>[2x]HHHHHHMASSAQDGNNPLFSPYKMGKFNLSHRVVLAPMTRCRALNNIPQAALGEYYEQRATAGGFLITEGTMISPTSAGFPHVPGI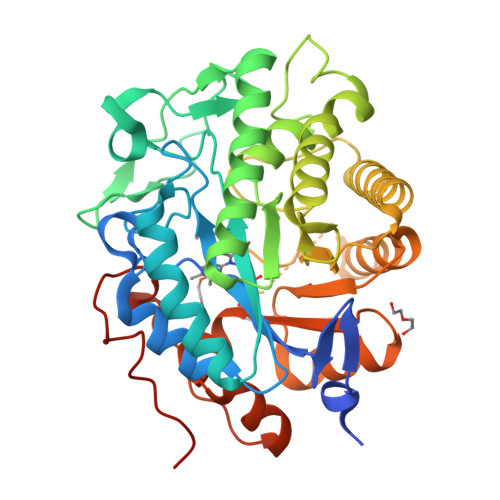FTKEQVREWKKIVDVVHAKGAVIFCQLWHVGRASHEVYQPAGAAPISSTEKPISNRWRILMPDGTHGIYPKPRAIGTYEISQVVEDYRRSALNAIEAGFDGIEIHGAHGYLIDQFLKDGINDRTDEYGGSLANRCKFITQVVQAVVSAIGADRVGVRVSPAIDHLDAMDSNPLSLGLAVVERLNKIQLHSGSKLAYLHVTQPRYVAYGQTEAGRLGSEEEEARLMRTLRNAYQGTFICSGGYTRELGIEAVAQGDADLVSYGRLFISNPDLVMRIKLNAPLNKYNRKTFYTQDPVVGYTDYPFLQGNGSNGPLSRL>[2x]GSHMTPISQTPGLLAEAMVDLGAIEHNVRVLREHAGHAQLMAVVKADGYGHGATRVAQTALGAGAAELGVATVDEALALRADGITAPVLAWLHPPGIDFGPALLAD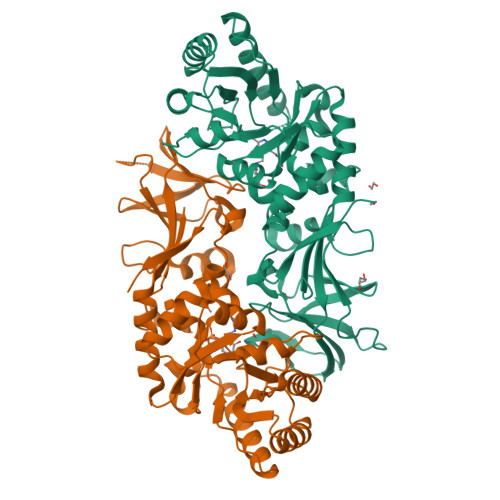VQVAVSSLRQLDELLHAVRRTGRTATVTVKVDTGLNRNGVGPAQFPAMLTALRQAMAEDAVRLRGLMSHMVYADKPDDSINDVQAQRFTAFLAQAREQGVRFEVAHLSNSSATMARPDLTFDLVRPGIAVYGLSPVPALGDMGLVPAMTVKCAVALVKSIRAGEGVSYGHTWIAPRDTNLALLPIGYADGVFRSLGGRLEVLINGRRCPGVGRICMNQFMVDLGPGPLDVAEGDEAILFGPGIRGEPTAQDWADLVGTIHYEVVTSPRGRITRTYREAENR>[18x]MAMKAYSMLNVTATLDGRRVIGLMDGDDAITTSPGVDVGTMLVGADGSWLFSQTADKSATVVIKLKPNSPTHRQLTEKWMAQRAGRLVGFPFDFIDSASNEGGTGAEFFIQKAPDDSKGNNAVVREWTIVTGEWTPTIPTLL;>MIDVAIAIDAESVEVTWRNRSGGSYDSRGNATGASWADTQIRAAIQPVSGRELQDLPEGVRSKVTLVAWTRSEVAENDQIIYLGDAYRVYAARPRPMDGFTRIALGKVSP[6x];>[6x]MRRITGITVIKDHQSEDRPALPYGVVELANFRDLHQQVRTIHYEDIEDSDNGEGFPEVQATPEVEQEWVFLVQVYGPGGLDYLRKVAAAFHVNQVNDLPGSLVIHEVAQINS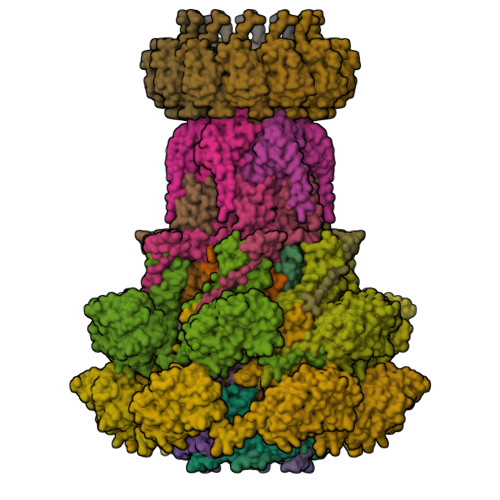IPEFLGERWEKRAQTNITLRGMSTDGFKVDVIEQHVINVTGERA;>[12x]MAKLPYSRVTNVTLTRTDNFPTRRGFGTQLILTHTAVSGQVDATKRTKLYASLAEVEADYPANTSVYKAALSAFSQNPRPIRLKVGYAATPTGGDDAAKKADFITSLGAILNYDQAFYQITLDAALRDQPYLDGLVEWVEAQPKIAMIDSNAAGHEDPANTTVIAARHKGTVERTAVFYHTDSTEYLAASMAAYMSTRVFDDANSAYTLKFKKAPGVRAIDKGSAVVTAITGFVEQTGQSESAGHCANTLIDIGDQEFLVEGSTLTQNVFLDEIHATDWIIARTEEEMLSLFLNNDRVPFTDQGMQQLASVPRAIMQLAARAGIVALDLNPLTGAYEPAYTITVPSVFDIPESQRKARIAPAIQVRFRYAGAVHYSVINYTMTF;>MNPIPAASDLKTRYPEFTGVSDAVVNAIIAEVNGMVDDGWEVSDQKPAVLALAAHMLSREGYPGRATNPNSFDPTNRPILSRKVGDVSTTFGRTDGGAAEGGANSYNYSSTVYGQTFLRLLRLNAPAVGLV[12x]>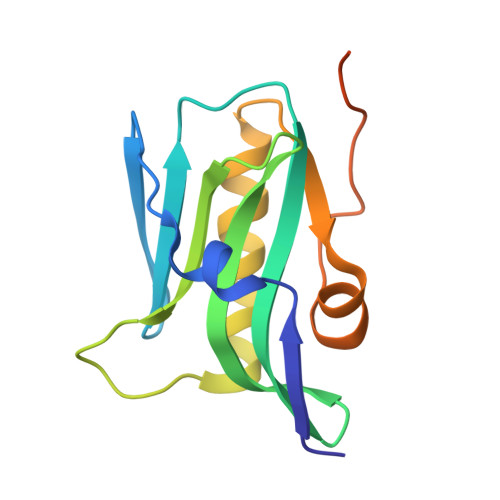 ASRYLTDMTLEEMSRDWFMLMPKQKVAGSLCIRMDQAIMDKNIILKANFSVIFDRLETLILLRAFTEEGAIVGEISPLPSLPGHTDEDVKNAVGVLIGGLERNDNTVRVSETLQRFAWRSSNENGRPPLPPKQKRKMARTIKSEV> MSTGDFLTKGIELVQKAIDLD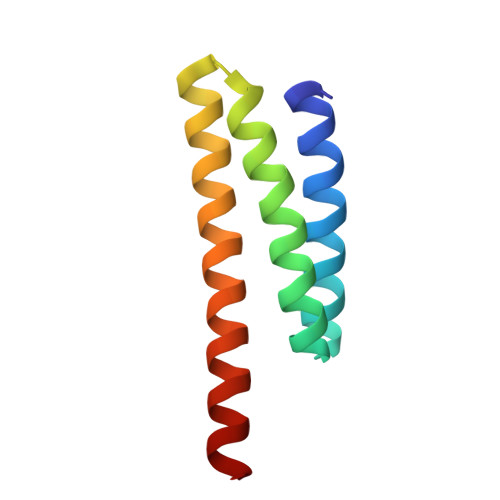TATQYEEAYTAYYNGLDYLMLALKYEKNPKSKDLIRAKFTEYLNRAEQLKKHLESEEANAA> EFNPYQKGPDPTASALERNGPFAIRSTSVSRTSVSGFGGGRLYYPTASGTYGAIAVSPGFTGTSSTMTFWGERLASHGFVVLVIDTITLYDQPDSRARQLKAALDYLATQNGRSSSPIYRKVDTSRRAVAGHAMGGGGSLLAARDNPSYKAAIPMAPWATSSTAFRTVSVPTMIFGCQDDSIAPVFSSAIPIYNAIPNSTRKNYVEIRNDDHLCVMNGGGHDATLGKLGISWMKRFVDNDTRYSPFVCGAEYNRVVS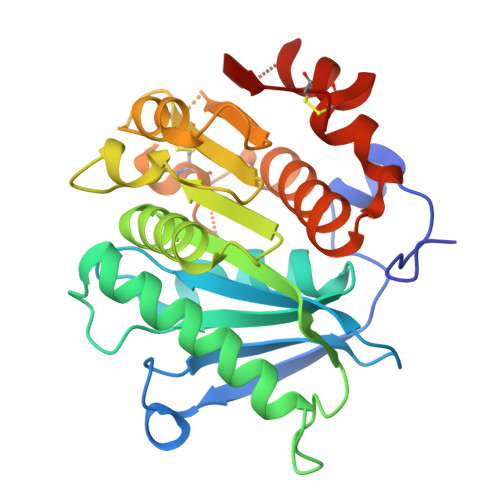SYEVSRSYNNCPY Supporting these invasion events are binary complexes formed between the apical membrane antigen (AMA) and rhoptry neck protein 2 (RON2) families that anchor the junction between parasite and host cell. Specifically, RON2s are transmembrane proteins secreted by apicomplexans into the host cell, integrated into the outer membrane, and presented on the host cell surface to serve as ligands for AMA proteins on the parasite surface. Toxoplasma gondii AMA1 adopts a stacked three domain architecture, with Domain I (DI) membrane distal and Domain III (DIII) membrane proximal. The apical surface is comprised of several loops from DI framing an apical groove, and a single extended loop from DII (DII loop) that packs against the side of DI and is stabilized by three tryptophan anchors buried into pockets on the TgAMA1 apical surface.

Most strikingly, EtRON2D3 bound approximately 275 fold tighter to TgAMA1ΔDIIloop (8.0 nM or greater) relative to TgAMA1 (2.2 μM). The 2.20 Å resolution crystal structure of TgAMA1ΔDIIloop in complex with EtRON2D3 showed clear electron density for the peptide seated in the apical groove. Three complexes in the asymmetric unit showed little variation in overall structure (TgAMA1ΔDIIloop: 0.32/0.60 Å rmsd over 392/387 Cα, chain A compared to C/E; EtRON2D3: 0.23/0.32 Å rmsd over 39/39 Cα, chain B compared to D/F), although an O-linked glycosylation on Thr425 of the DII-DIII linker was modelled only in chain A. Since EtRON2D3 chain D showed the lowest thermal motion, the TgAMA1ΔDIIloop chain C complex with EtRON2D3 chain D was used for further analyses unless otherwise noted. EtRON2D3 bound throughout the apical groove of TgAMA1ΔDIIloop in the expected conformation based on previous AMA1-RON2 co-structures, with the EtRON2D3 N-terminal helix seated in the area exposed by the absence of the TgAMA1 DII loop, followed by a length of ordered coil, a beta-hairpin loop, and ordered C-terminal coil that extends back through the apical groove. In contrast to previously characterized AMA1-RON2 complexes, the electron density surrounding the cysteine residues of EtRON2D3 (Cys1278 and Cys1288) revealed a population with only a partially formed disulfide bond. While the second cysteine (Cys1288) was appropriately positioned to form the disulfide, density based refinement of the occupancy for the first cysteine (Cys1278) showed 41 to 74% oriented away from the central axis of the disulfide bond (inset). An initial comparison of the TgAMA1-TgRON2D3 and TgAMA1ΔDIIloop-EtRON2D3 interfaces revealed similar overall buried surface areas (~3400 Å2 for each complex), but an overlay of the TgRON2D3 peptide on the TgAMA1ΔDIIloop-EtRON2D3 complex shows key areas of divergence. Most importantly, the N-terminal helix adopts a different angle between the two peptides, the coil leading up to the first cysteine is restructured, and the tip of the cystine loop is shifted.

>[3x]GSAMGSASTSGNPFQANVEMKTFMERFNLTHHHQSGIYVDLGQDKEVDGTLYREPAGLCPIWGKHIELQQPDRPPYRNNFLEDVPTEKEYKQSGNPLPGGFNLNFVTPSGQRISPFPMELLEKNSNIKASTDLGRCAEFAFKTVAMDKNNKATKYRYPFVYDSKKRLCHILYVSMQLMEGKKYCSVKGEPPDLTWYCFKPRKSVTENHHLIYGSAYVGENPDAFISKCPNQALRGYRFGVWKKGRCLDYTELTDTVIERVESKAQCWVKTFENDGVASDQPGSGSGSGDQPHSGGVGRNYGFYYVDTTGEGKCALSDQVPDCLVSDSAAVSYTAAGSLSEETPNFIIPSNPSVTPPTPETALQCTADKFPDSFGACDVQACKRQKTSCVGGQIQSTSVDCTADEQNECGSNTAAALVPR;>GSASDITQHLNDSGLGPAVECLENLVVGPVCPAAVVAPAV[3x]>[2x]MELKNSI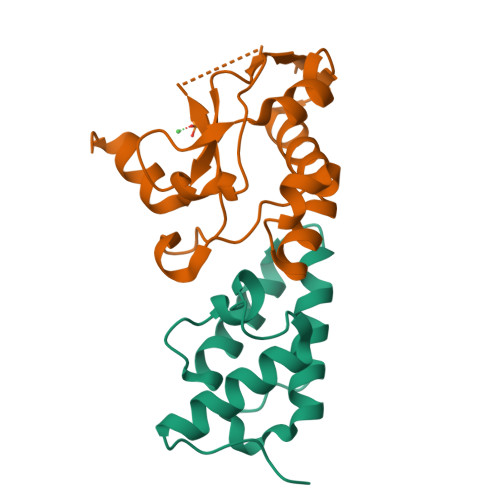SDYTEAEFVQLLKEIEKENVAATDDVLDVLLEHFVKITEHPDGTDLIYYPSDNRDDSPEGIVKEIKEWRAANGKPGFKQGHHHHHH;>MESKRNKPGKATGKGKPVNNKWLNNAGKDLGSPVPDRIANKLRDKEFKSFDDFRKKFWEEVSKDPELSKQFSRNNNDRMKVGKAPKTRTQDVSGKRTSFELHEEKPISQNGGVYDMDNISVVTPKRHIDIHRGK[2x]3H-imidazo[2,1-b]purin-4(5H)-one | 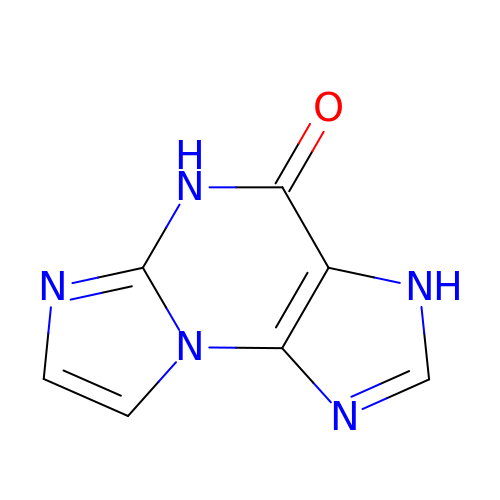C7 H5 N5 O | OSXKHFTZRHDUJN-UHFFFAOYSA-N> MGATKILMDSTHFNEIRSIIRSRSVAWDALARSEELSEIDASTAKALESILVKKNIGDGLSSSNNAHSGFKVNGKTLIPLIHLLSTSDNEDCKKSVQNLIAELLSSDKYGDDTVKFFQEDPKQLEQLFDVSLKGDFQTVLISGFNVVSLLVQNGLHNVKLVEKLLKNNNLINILQNIEQMDTCYVCIRLLQELAVIPEYRDVIWLHEKKFMPTLFKILQRATDSQLATRIVATNSNHLGIQLQYHSLLLIWLLTFNPVFANELVQKYLSDFLDLLKLVK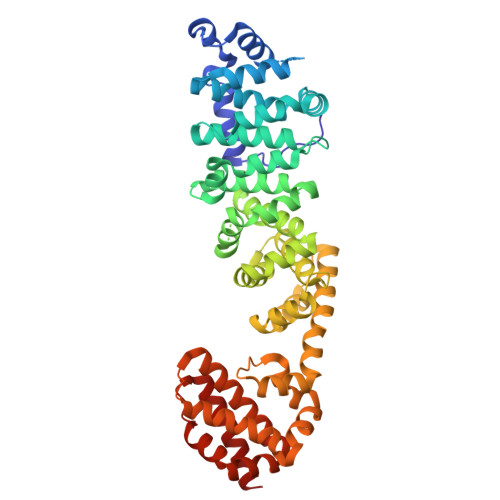ITIKEKVSRLCISIILQCCSTRVKQHKKVIKQLLLLGNALPTVQSLSERKYSDEELRQDISNLKEILENEYQELTSFDEYVAELDSKLLCWSPPHVDNGFWSDNIDEFKKDNYKIFRQLIELLQAKVRNGDVNAKQEKIIIQVALNDITHVVELLPESIDVLDKTGGKADIMELLNHSDSRVKYEALKATQAIIGYTFK>[2x]MSANDLPRGPEEGAPERKTREKPSQEQTDWSGSFSAYLESHRASLVDSLRRLFGHPFGSFFTCLVMGITLSLPMGLSLLLNNVERLGGSWQRAAQISLFLDLKTSENQGQDLREQIERLPDVIEAQLISREQALSELQEQSGLGEALKELPENPLPPVISVTPKQIDRAGLEALRQQLAELPHVQQAQLDLVWVERLSAILKLGERFVFGLTILLVLTLLLVVGNTIRLHIENRRNEIEVIKLVGGTDGYVRRPFLYMGALYGLGAGILSWALLAYSLNWLNGSVVNLSGLYGSDFGLQGVPLDDGLSLTVGAVLLGWVGAWLAVARHLRELAPR;>MIRFEQVG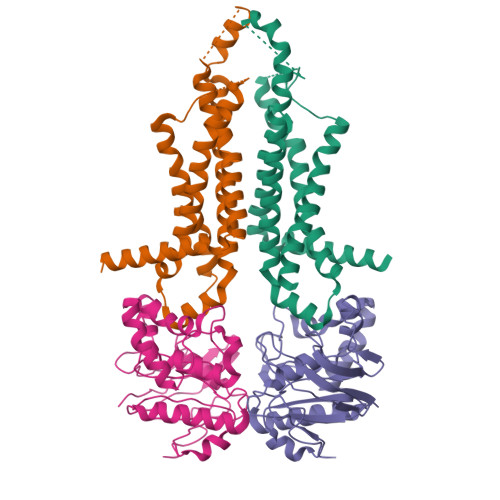KRYPNGHVGLHEVSFRVHRGEILFVTGHSGAGKSTLLRLILAMERPTSGKLLLGGQDLGRITTAQIPFLRRQIGVVFQNHQLLTDRTVADNIALPLQILGMPKPEIAKRVASALERVNLKEKGEALPSDLSTGQQQRVGIARAIVHQPALLLADEPTGNLDPRLASEIMGVFEDINRLGTTVLIASHDLALIARMRHRMLTLQRGRIIADREDEA[2x]> HHHHHHDYKDDDDKLEVLFQGPEFRNEIRQKINPYRSHMKQKFQVLWEKEPCLLVPEDFYEETTKIEYELLSTVYLDAFKPGESSPTVVLHGPEGIGKTTFLRKVMLEWAKGNLWRDRFSFVFFLTGREMNGVTDMSLVELLS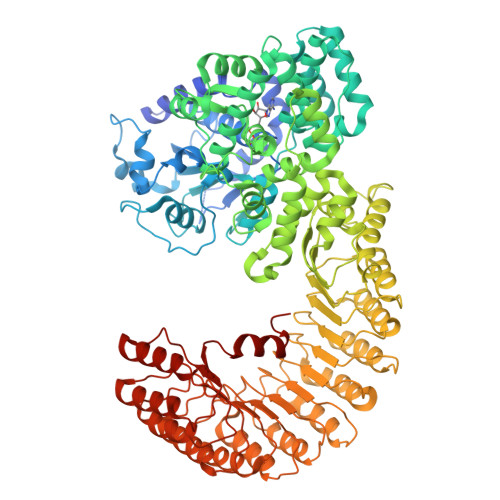RDWPESSEPIEDIFSQPERILFILDGMEELKFDLDCNADLCEDWEQPQSMQVVLQSLLQKQMLPECSLLLALSKMGMRKNYSLLKHMKCIFLLGFSEHQRKLYFSHYFQEKDASSRAFSFVREKSSLFVLCQSPFLCWLVCTSLKCQLEKGEDLELDSETITGLYVSFFTKVFRSGSETCPLKQRRARLKSLCTLAAEGMWTCTFLFCPEDLRRNGVSESDTSMWLDMKLLHRSGDCLAFIHTCIQEFCAAMFYMFTRPKDPPHSVIGNVTQLITRAVSGHYSRLSWTAVFLFVFSTERMTHRLETSFGFPLSKEIKQEITQSLDTLSQCDPNNVMMSFQALFNCLFETQDPEFVAQVVNFFKDIDIYIGTKEELIICAACLRHCHSLQKFHLCMEHVFPDESGCISNTIEKLTLWRDVCSAFAASEDFEILNLDNCRFDEPSLAVLCRTLSQPVCKLRKFVCNFASNLANSLELFKVILHNPHLKHLNFYGSSLSHMDARQLCEALKHPMCNIEELMLGKCDITGEACEDIASVLVHNKKLNLLSLCENALKDDGVLVLCEALKNPDCALEALLLSHCCFSSAACDHLSQVLLYNRSLTFLDLGSNVLKDEGVTTLCESLKHPSCNLQELWLMNCYFTSVCCVDIATVLIHSEKLKTLKLGNNKIYDAGAKQLCKALKHPKCKLENLGLEACELSPASCEDLASALTTCKSLTCVNLEWITLDYDGAAVLCEALVSLECSLQLLGLNKSSYDEEIKMMLTQVEEMNPNLIISHHLWTDDEGRRRGILV> CIKCDQFVTDALKTFENTYLNDHLPHDIHKNVMRMVNHEVSSFGVVTSAEDSYLGAVDENTLEQATWSFLKDLKRITDSDLKGELFIKELLWMLRHQKDIFNNLARQFQKEVLCPNKCGVMSQTLIWCLKCEKQLHICRKSLDCGERHIEVHRSEDLVLDCLLSWHRASKGLTDYSFYRVWENSSETLIAKGKEPYLTKSMVGPEDAGNYRCVLDTINQGHATVIRYDVTVLPPKH

In mammals this process critically depends on the interaction between Izumo1, a protein exposed on the equatorial segment of acrosome-reacted sperm, and the egg plasma-membrane-anchored receptor Juno 1, 2. Juno and Izumo are structurally unrelated: Juno adopts a modified folate receptor family fold, whereas Izumo1 is a type I transmembrane protein consisting of an extracellular region of about 300 residues and a short cytoplasmic tail. Izumo1 is not considered a fusogen per se because it cannot induce membrane fusion when heterologously expressed in commonly used cell lines. The molecular mechanism triggering gamete fusion is unresolved because both Izumo1 and Juno lack sequence similarity to known membrane fusogens.

Here we report the crystal structure of Izumo1, which reveals a membrane distal region composed of a four-helix bundle connected to a carboxy-terminal immunoglobulin (Ig)-like domain through a β-hairpin stabilized by disulfide bonds. The structure shows that the Izumo domain consists of a four-helix bundle with a flexible α-helical hook/β-sheet insertion, followed by a β-hairpin that connects the bundle to a seven-stranded Ig-like domain. These features result in an elongated architecture stabilized by five intramolecular disulfide bonds that are conserved in the three Izumo paralogs, and are clearly discernible within the sequence of Spaca6, another sperm surface protein recently reported to be required for gamete fusion. The helical character of the carboxy-terminal half of the Izumo domain, which corresponds to helices α3 and α4 in our structure, was shown to be important for the function of Izumo1. The structure readily explains why mutation of leucine residues to proline interferes with this biological activity by disrupting the fold of the four-helix bundle. Strikingly, structural homology searches revealed a high confidence match between the four-helix bundle of Izumo1 and that of SPECT1, a secreted Plasmodium protein that is essential for host cell traversal by the infective sporozoite form of the parasite (Dali Z-score 6.9, RMSD 3.3 Å over 98 residues). In addition, the β-hairpin of Izumo1 is structurally similar to the extensible β-ribbon of TRAP, another Plasmodium protein that mediates sporozoite gliding and host cell invasion (RMSD 1.4 Å over 19 residues). The presence of solvent-exposed bulk aromatic residues in the Izumo1 four-helix bundle (a feature also observed in SPECT1) and the report that some monoclonal antibodies that target the Izumo domain do not block binding of sperm to the egg but hinder gamete fusion are consistent with the possibility that an additional, as yet unknown, component is required to form a functional fusogenic complex. Our findings suggest that the four-helix bundle of the Izumo domain and SPECT1 may orchestrate analogous fusion-related molecular recognition events at the sperm–egg and parasite–host cell interfaces.3-ethoxybenzoic 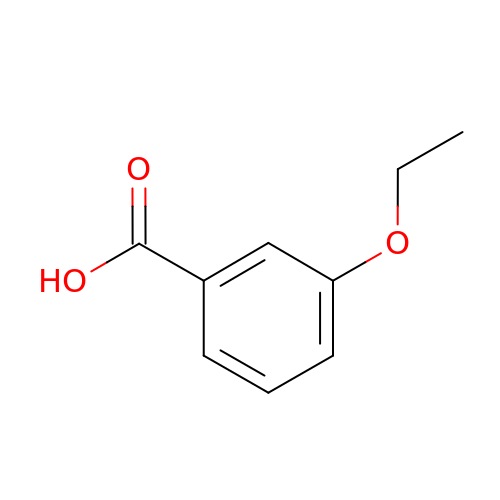acid | C9 H10 O3 | DTFQMPQJMDEWKJ-UHFFFAOYSA-N> MEHVAFGSEDIENTLAKMDDGQLDGLAFGAIQLDGDGNILQFNAAEGDI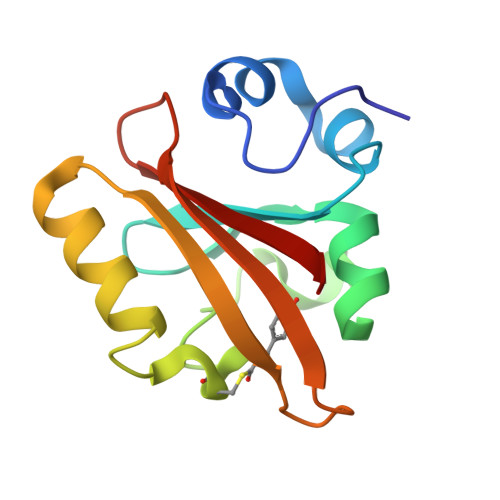TGRDPKQVIGKNFFKDVAPCTDSPEFYGKFKEGVASGNLNTMFEYTFDYQMTPTKVKVHMKKALSGDSYWVFVKRV> MKKQTQLLSALALSVGLTLSASFQAVASIPGQVADQAPLPSLAPMLEKVLPAVVSVRVEGTASQGQKIPEEFKKFFGDDLPDQPAQPFEGLGSGVIINASKGYVLTNNHVINQAQKISIQLNDGREFDAKLIGSDDQSDIALLQIQNPSKLTQIAIADSDKLRVGDFAVAVGNPFGLGQTATSGIVSALGRSGLNLEGLENFIQTDASINRGNAGGALLNLNGELIGINTAILAPGGGSVGIGFAIPSNMARTLAQQLIDFGEIKRGLLGIKGTEMSADIAKAFNLDVQRGAFVSEVLPGSGSAKAGVKAGDIITSLNGKPLNSFAELRSRIATTEPGTKVKLGLLRNGKPLEVEVTLDTSTSSSASAEMITPALEGATLSDGQLKDGGKGIKIDEVVKGSPAAQAGLQKDD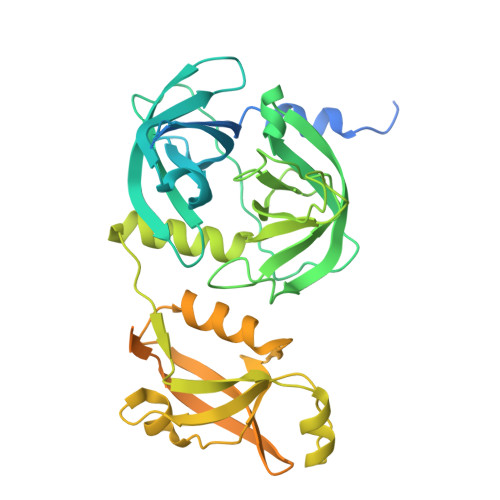VIIGVNRDRVNSIAEMRKVLAAKPAIIALQIVRGNESIYLLMRLWHHHHHH>[13x]SNAMAAGGPGAGSAAPVSSTSSLPLAALNMRVRRRLSLFLNVRTQVAADWTALAEEMDFEYL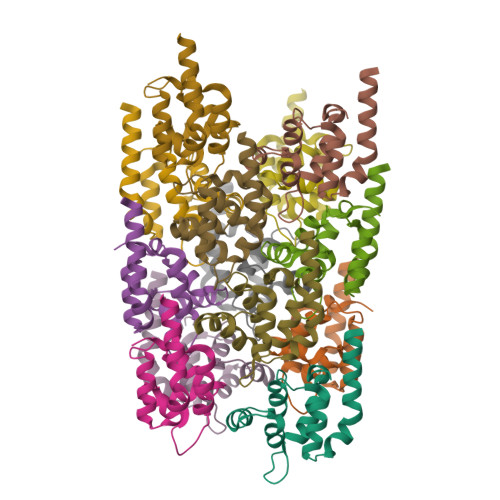EIRQLETQADPTGRLLDAWQGRPGASVGRLLELLTKLGRDDVLLELGPSIEEDCQKYILKQQQEEAEKPLQVAAVDSSVPRTAELAGITTLDWSHPQFEK> GGCUUAUCAAGAGAGGGGGAGCGACUGGCGCGAAGAGCCCCGGCAACCAGAAAUGGUGCCAAUUCCUGCAGCGGAAACGUUGAAAGA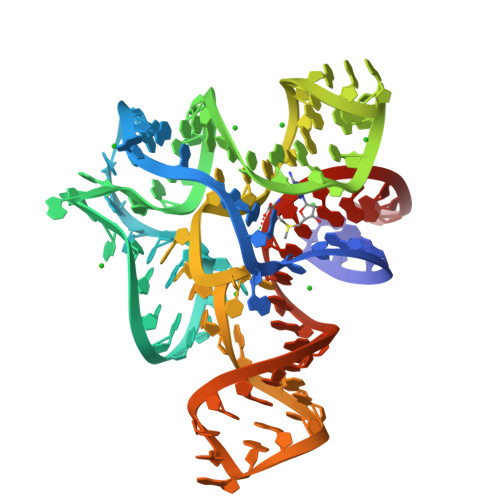UGAGCCG> GPDSMAPPVRYCIPGERLCNLEEGSPGSGTYTRHGYIFSSLAGCLMKSSENG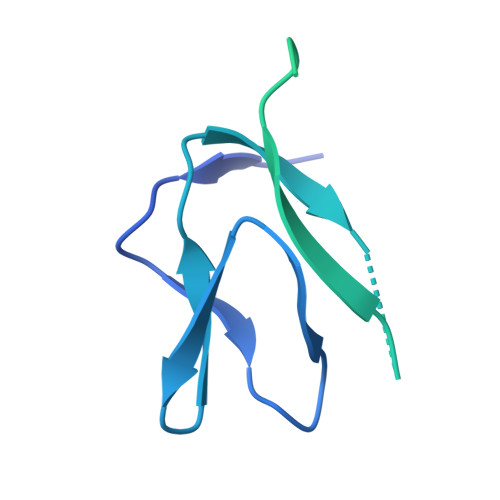ALPVVSVVRETESQLLPDVGAIVTCKVSSINSRFAKVHILYVGSMPLKNSFRGTIRKEDVRATEKDKVEIYKSFRPGDIVLAKVISLGDAQSNYLLTTAENELGVVVAHSESGIQMVPISWCEMQCPKTHTKEFRKVARVQPEFLQT>[3x]NSSSLNVDGRSSKQHGKRDSKITDHFVRIPKSEDKRKEQCEVRHQRAERKIPKYVPPNLPPDKKWLGTPIEEMRKMPRCGVRLPLLRPSASHTVTVRVDLLRAGEVPKPFPTHYKDLWDNKHVKMPCSEQNLYPVEDENGERTAGSRWELIQTALLNKFTRPQNLKDAILKYNVAYSKKWDFTALVDFWDKVLEEAEAQHLYQSILPDMVKIALCLPNICTQPIPLLKQKMNHSVTMSQEQIASLLANAFFCTFPRRNAKMKSEYSSYPDINFNRLFEGRSSRKPEKLKTLFCYFRRVTEKKPTGLVTFTRQSLEDFPEWERCDKPLTRLHVTYEGTIEGNGRGMLQVDFANRFVGGGVTGAGLVQEEIRFLINPELIVSRLFT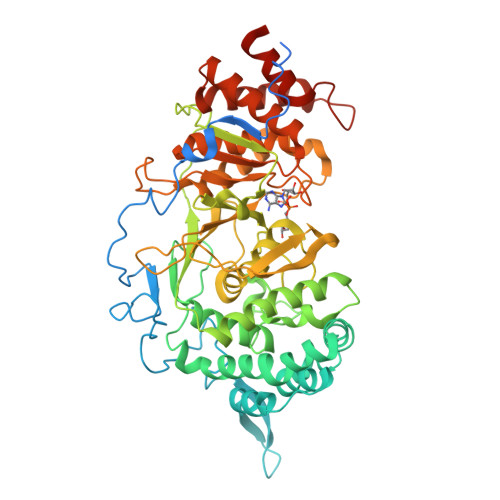EVLDHNECLIITGTEQYSEYTGYAETYRWARSHEDGSEKDDWQRCCTEIVAIDALHFRRYLDQFVPEKVRRELNKAYCGFLRPGVPPENLSAVATGNWGCGAFGGDARLKALIQLLAAAAAERDVVYFTFGDSELMRDIYSMHTFLTERKLNVGKVYRLLLRYYREECRDCSSPGPDTKLYPFIYHAAESSAETSDQPGQRTGT>GSHMHRVINHPYYFPFNGKQAEDYLRSKERGDFVIRQSSRGDDHLAITWKLDKDLFQHVDIQELEKENPLALGKVLVVEGQRYHDLDQIIVEYLQNKIRLLNELTSNEKFKAGTKKEVVKFIEDYSKVNPKKSVYYFSLNYENPGWFYLIFKLNAESKLYIWNVKLTHTGFFLVNYNYPTVIQLCNGFKT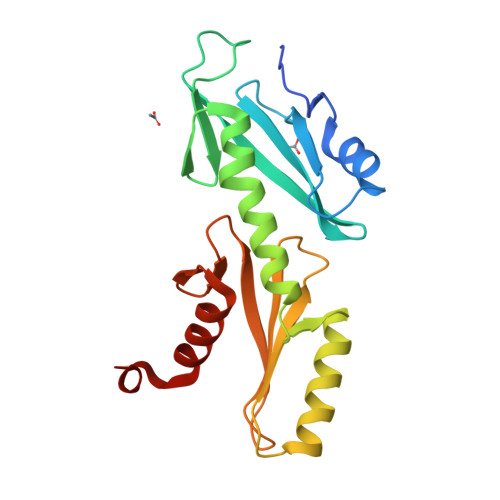LLKSSNTRN[2x]> MARASEKGEEKKQSNN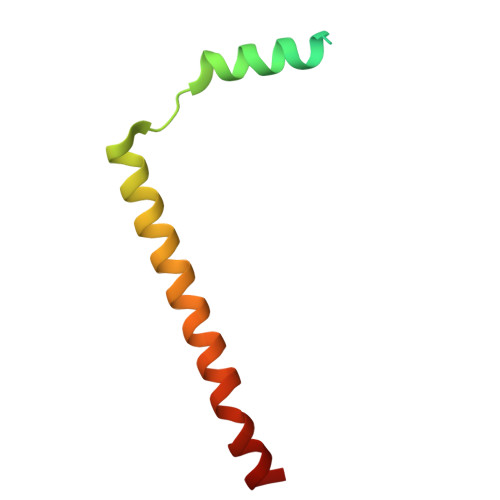QVEKLVEAPVEFVREGTQFLAKCKKPDLKEYTKIVKAVGIGFIAVGIIGYAIKLIHIPIRYVIV Oligoribonucleases (Orns) are highly conserved DnaQ-fold 3′-5′ exoribonucleases that have been found to carry out the last step of cyclic-di-GMP (c-di-GMP) degradation, that is, pGpG to GMP in several bacteria. Orns are highly conserved DnaQ-fold 3′-5' exoribonucleases with a DEDDh active site motif that degrade short 2- to 5-mer oligoribonucleotides in 3′-5' direction and release monoribonucleotides as reaction products. Removal of pGpG is critical for c-di-GMP homeostasis, as excess uncleaved pGpG can have feedback inhibition on phosphodiesterases, thereby perturbing cellular signaling pathways regulated by c-di-GMP. Removal of pGpG is important to maintain the pool of free nucleotides inside the cell and to prevent mispriming of transcripts and is brought about by Orns.

In order to obtain better understanding of the additional C-terminal helix, α10, in Ms_orn, the structure of Orn of Escherichia coli (Eco_orn) with the canonical Rnase-H fold was also determined for comparative structural analysis. The final structure of Eco_orn could be traced from residues 2 to 181 of the polypeptide chain. Eco_orn was also identified as a dimer by gel filtration, SEC–MALLS and PISA. Superposition of Eco_orn structure over Ms_orn indicates overall structural similarity with rmsd of 1.134 Å across 347 Cα-atoms of the dimer but lacking the C-terminal tail of Ms_orn. Eco_orn, on the other hand, buries only 17.2% of total solvent-accessible area comprising nearly 1650 Å2 in the dimer interface. The nature and position of residues forming H-bonds at the interface is similar in both proteins. Interestingly, estimated Tm (50 °C) of Eco_orn (which naturally lacks the C-terminal extended region) was similar to that of Ms_ornΔC, suggesting α10 aids the higher observed thermostability of Ms_orn (under mild denaturing conditions). The denaturation curve of Eco_orn shows a monophasic manner of transition from folded to unfolded state, whereas both mycobacterial proteins exhibit a biphasic transition. Quantum yield of ANS fluorescence for Eco_orn at its native state in the absence of Gdm-HCl, on the other hand, itself is two-fold higher than that of its fully denatured state, suggesting that native Eco_orn has partially exposed hydrophobic surfaces, whereas Ms_orn is more tightly packed. Once again, Eco_orn, naturally lacking the C-terminal extended region, appears to follow a different unfolding pattern from Ms_orn when monitored by either changes in λmax of intrinsic fluorescence or [θ]222 nm, suggesting that the unfolding pathways of Ms_orn with the extended C-terminal tail are different from other Orns.

>SMSANENNLIWIDLEMTGLDPERDRIIEIATLVTDANLNILAEGPTIAVHQSDEQLALMDDWNVRTHTASGLVERVKASTMGDREAELATLEFLKQWVPAGKSPICGNSIGQDRRFLFKYMPELEAYFHYRYLDVSTLKELARRWKPEILDGFTKQGTHQAMDDIRESVAELAYYREHFIKL[4x]> CPPRHFKVGTMSSCSPWLKCPEIRSGVRRVKLIGQGAVKKVYLSEWQGQKVALSVLSSDQYADDFLHGLSMLRALQSSHVVTLVGVCEED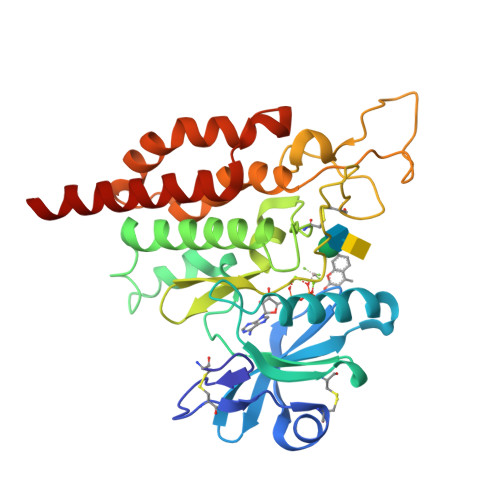AVFVTEYHPLGSVLTLDTTLAQERYRWRNSWHTRLQLAIDYVAFLAYLHSSPAGIRVMCDSNDLHKTLSQFLLASDMRLLANDLDALPEVEKGGLGVKCGHHELTGDFVAPEQLWPYGEDFSFSDEAMPGYDEKTDIWKIPDVTRFLLGDVLGGDVIHFHLFQIYSECKRKEAHMRPTAREVLSVYRSVYDSMMESQSQR> DYRSPFIASVSDQHGVVYITENKNKTVVIPCLGSISNLNVSLCARYPEKRFVPDGNRISWDSKKGFTIPSYMISYAGMVFCEAKINDESYQSIMYIVVVVGYRIYDVVLSPSHGIELSVGEKLVLNCTARTELNVGIDFNWEYPSSKHQHKKLVNRDLKT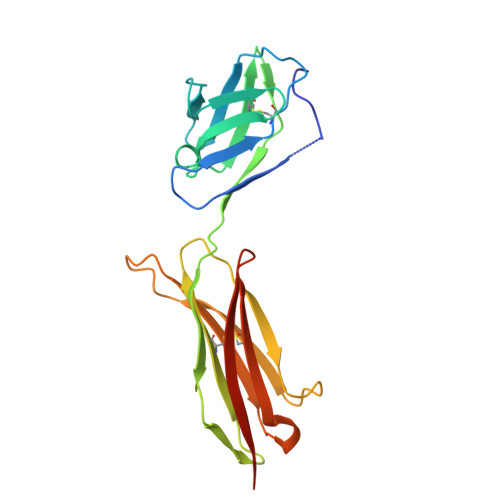QSGSEMKKFLSTLTIDGVTRSDQGLYTCAASSGLMTKKNSTFVRVHEDPIEGR> GPLGSPEFPGGIWNTLLAIHKTEKAVETPKKVFAVANGVLYSVGKEAPHEAKIFDRISGLSDTSVSSIAYSEQLKSLVIYYASGNIDILDEAGRVTNVPALKDNIDLIDKTLNRLLIVGNRAYLAGGFGLSVLDVAEARIPATYAKGTKVTDVAKLDNDRLLMLKEGQLFIGKETDNLQDPAAWTALSLNLPMGSVTGLGIVGEDICFLLADGRVYVAANQSFEPELLLSSSADSRLYVTDRGLFICAENRIYFIEKGRKTTQFPIADVLGVGAMNESNTAYIALGEEGLASLLLAEGSTAEAMPVAFDGPGDNDFYEMRFSHGRLYAASGLWGTNLMGHAGMVKLYDGNRWTNFDKKTVQEQLGGGFSFNDAIDIAVSNGDPDHFFVGTWGNGLFEFKDGKAIARYSGNETAIAECNPGDARVKAIAFDNKGNLWGTLGAVGKNIFMYDPQSSTWHSFSYPDVANLASFGNMIILPNGDKWVNILHRSGGSTRKGVLIFNDRGTPETTSDDSHLYVEQFVNRLGAAIGHKTIYAMAVDHNGSVWMGSDIGIFGVYNAAGVLSSTSTPIAVRPVGGEEPNLYYVLDKVTVTDIVVDKLNHKWVATQGTGLYLLSEDCSKILAQFTVENSPLLSNNILSLALNDDNGLLYIGTADGLMTFQTGTGSGSASELDGVYVYPNPLRPEYPDGVTIAGLQAGCSVKITDTTGRLLYQTESVTTEVKWNARGADGNRVASGVYAVAVYDPVSKKSKLIRFAVIR

The most recently discovered system of protein secretion is T9SS, also called Por secretion system, which operates exclusively in selected species within the Bacteroidetes phylum. T9SS is essential for the secretion of many proteinaceous virulence factors by P. gingivalis, and has, thus, attracted considerable attention as a possible target for pharmaceutical intervention to treat severe periodontal disease and restore homeostasis of the oral microbiome. Here, we discovered a new component of T9SS, PorZ, and found it loosely associated with the P. gingivalis cell surface in a manner independent of A-LPS anchorage. To sum up, the reported full molecular and functional characterization of PorZ, a novel essential surface component of T9SS, contributes to our understanding of protein secretion as part of host-microbiome interactions by dysbiotic members of the human oral cavity.

We produced PorZ without its predicted signal peptide (residues Q26-R776) by recombinant overexpression in Escherichia coli, and succeeded in crystallizing and solving its structure by single-wavelength anomalous diffraction with a selenomethionine derivative. The structure was refined with data to 2.9 Å resolution and consists of three domains. The first two are consecutive N-terminal seven-stranded β-propeller or circular-leaflet moieties (βD1: residues K39—M322; and βD2: G29—L34+Y335—T679 373839; PorZ residue numbering in superscript notation according to UP Q9S3Q8), each featuring a shallow cylinder or thick disk with an “entry side” and an “exit side”. These domains are succeeded by a C-terminal domain (CTD, V692—R776). The two propellers are offset from one another by a ~90° rotation about the intersection axis of the propellers’ planes. This causes the overall molecular structure to be reminiscent of an easy chair of approx. maximal dimensions 95 × 80 × 55 Å, with βD1 as the seat, βD2 the backrest, and CTD the backrest support. In the case of PorZ, which consists of two consecutive seven-fold propellers, the N-terminal segment of the polypeptide chain follows such a mechanism and forms strand βD2-VII-β4, while the remaining three strands of this blade are provided by the polypeptide chain after forming both propellers. Despite some general differences, in particular in loops, the architecture and strand connectivity is equivalent to that of the CTD of RgpB, which is the structural paradigm of a functional CTD required for T9SS secretion. Along this line, the crystal structure of PorZ revealed potential polyethylene glycol fragments bound at the hinge between βD1 and βD2 on their entry side, as well as on the exit surface of βD2.> MSLTDVMFKSQIANQLKNLRKSRGLSLDATAQLTGVSKAMLGQIERGESSPTIATLWKIASGLEASFSAFFANDPQLLSSERSFPDDLNMKIHTLFPYAADTGLEIFEITLLDHHQQMSSPHALGVIEYIHVLEGIMKVFFDEQWHELQQGEHIRFFSDQPHGYAAVTEKAVFQNIVAYPRR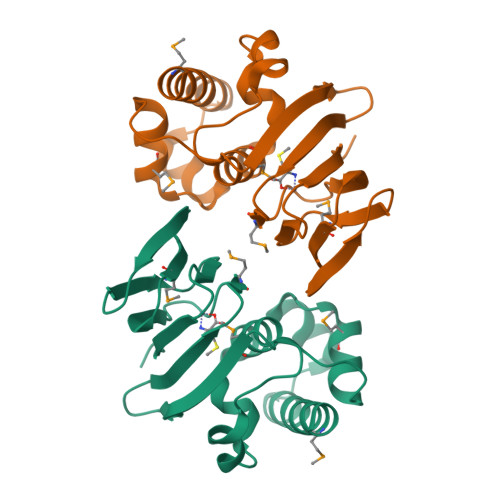EGGSHHHHHH benzyl hydroxycarbamate | C8 H9 N O3 | 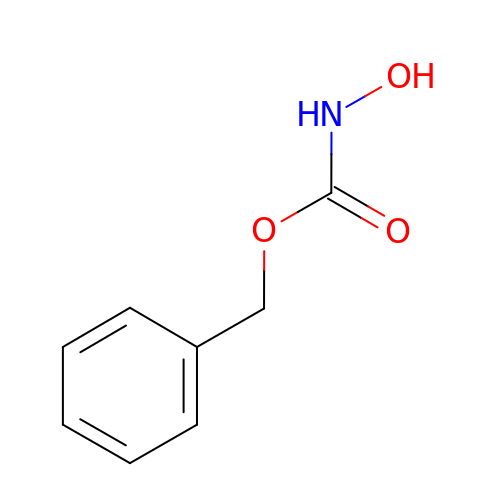PQBSPTAPCMSZAA-UHFFFAOYSA-N>[6x]GSHMDYNKRSSVSTVPNAAPIRVGFVGLNAAKGWAIKTHYPAILQLSSQFQITALYSPKIETSIATIQRLKLSNATAFPTLESFASSSTIDMIVIAIQVASHYEVVMPLLEFSKNNPNLKYLFVEWALACSLDQAESIYKAAAERGVQTIISLQGRKSPYILRAKELISQGYIGDINSIEIAGNGGWYGYERPVKSPKYIYEIGNGVDLVTT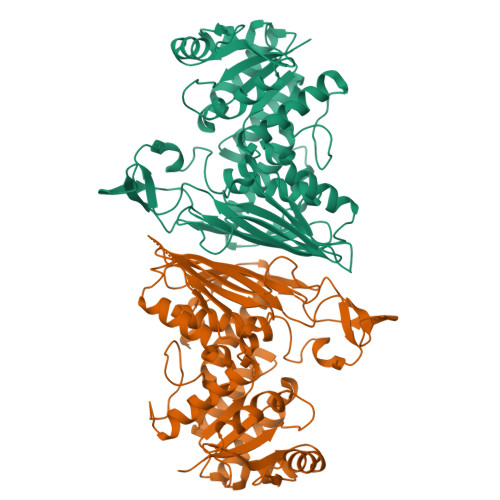TFGHTIDILQYMTSSYFSRINAMVFNNIPEQELIDERGNRLGQRVPKTVPDHLLFQGTLLNGNVPVSCSFKGGKPTKKFTKNLVIDIHGTKGDLKLEGDAGFAEISNLVLYYSGTRANDFPLANGQQAPLDPGYDAGKEIMKVYHLRNYNAIVGNIHRLYQSISDFHFNTKKIPELPSQFVMQGFDFEGFPTLMDALILHRLIESVYKSNMMGSTLNVSNISHYSL> XIWIAQEL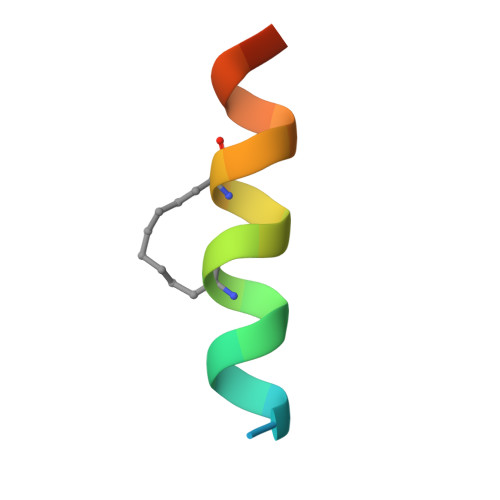RLIGDLFNAYYARR N-(3-chloro-2-methylphenyl)-4-(3,4-dimethyl-7-oxo-2-phenyl-2,7-dihydro-6H-pyrazolo[3,4-d]pyridazin-6-yl)butanamide 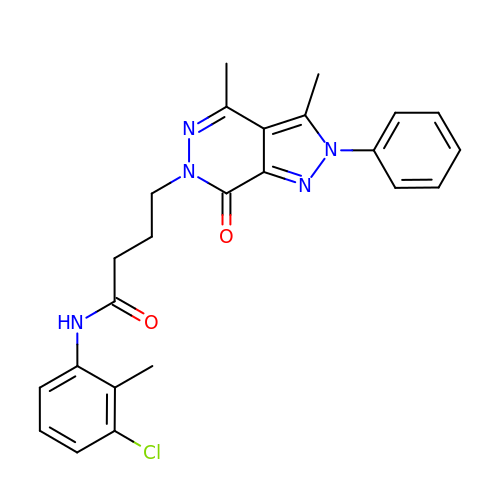| C24 H24 Cl N5 O2 | HPMUIOXFVVIJSJ-UHFFFAOYSA-N6-HYDROXY-6-METHYL-HEPTAN-3-ONE 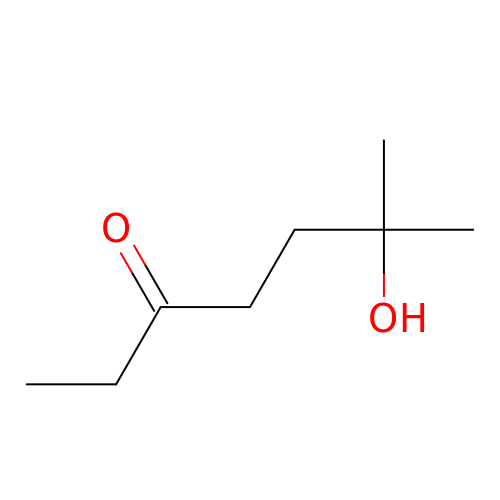| C8 H16 O2 | FGPMBONEKHYAHO-UHFFFAOYSA-N6-[4-(3-fluorobenzoyl)-1H-pyrrol-2-yl]-2-hydroxy-4-oxohexa-2,5-dienoic acid | C17 H12 F N 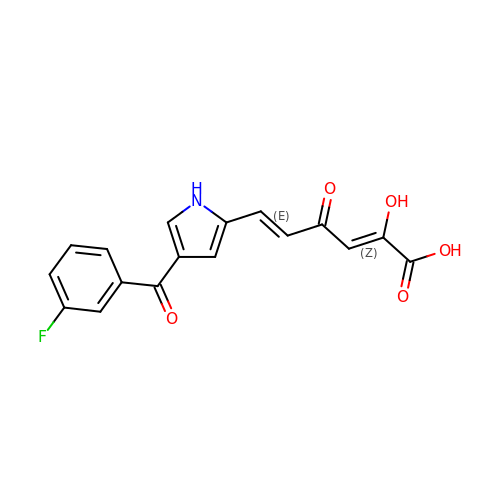O5 | WQEAOCAOIXLGFY-OQLOTXMNSA-N> SMQTFLKGKRVGYWLSEKKIKKLNFQAFAELCRKRGMEVVQLNLSRPIEEQGPLDVIIHKLTDVILEADQNDSQSLELVHRFQEYIDAHPETIVLDPLPAIRTLLDRSKSYELIRKIEAYMEDDRICSPPFMELTSLCGDDTMRLLEKNGLTFPFICKTRVAHGTNSH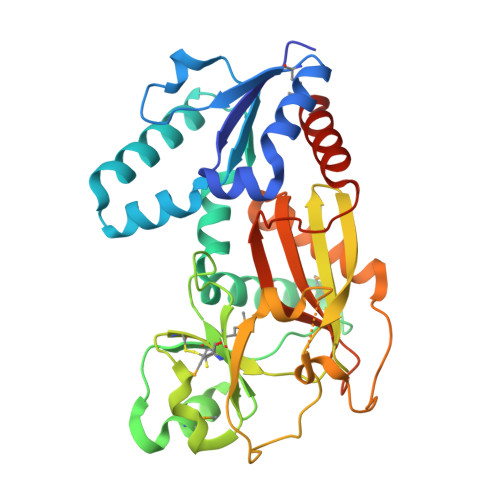EMAIVFNQEGLNAIQPPCVVQNFINHNAVLYKVFVVGESYTVVQRPSLKNFSAGTSDRESIFFNSHNVSKPESSSVLTELDKIEGVFERPSDEVIRELSRALRQALGVSLFGIDIIINNQTGQHAVIDINAFPGYEGVSEFFTDLLNHIATVLQGQSTAM> GSHMASNRTFSYTLEDHTKQAFGIMNELRLSQQLCDVTLQVKYQDAPAAQFMAHKVVLASSSPVFKAMFTNGLREQGMEVVSIEGIHPKVMERLIEFAYTASISMGEKCVLHVMNGAVMY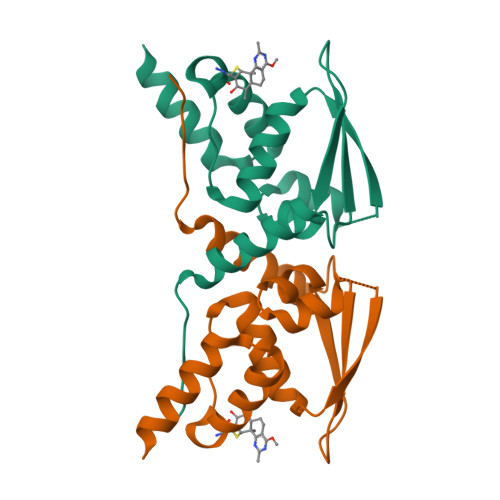QIDSVVRACSDFLVQQLDPS> MDRDQGASDNLLERKNILIASIMTSYRDLITHATSPITSAT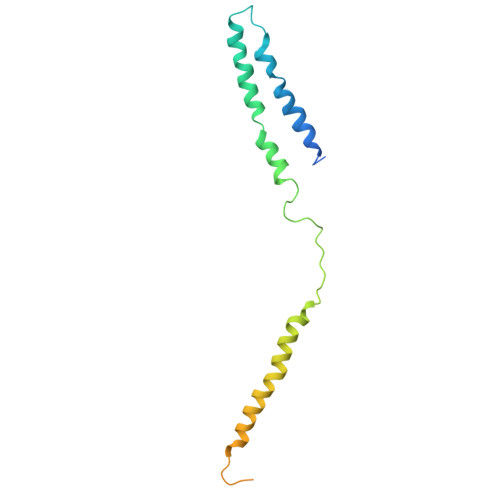ASPGHAGYSSMALSTAIHAAVKYTEDLLSLTRTLREALWVVGPLTGPGEKDAQAEEGMAKDAEVVWDVLNEMRDRERERMMAALMEGDTRVRGAVRFERGDVEVVVAGQGQQIEMGRGVNGEVKSEGA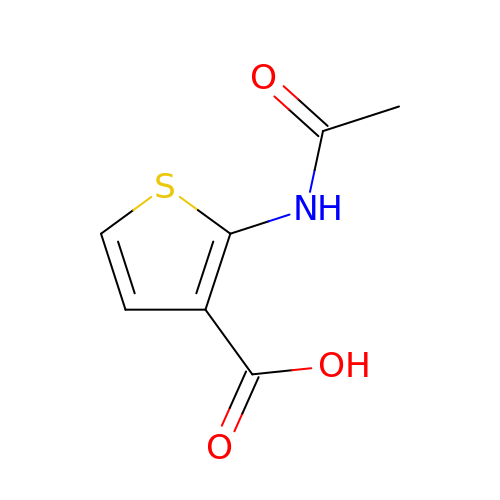2-(ACETYLAMINO)THIOPHENE-3-CARBOXYLIC ACID | C7 H7 N O3 S | RCEBHKDQZCVBTC-UHFFFAOYSA-N>[2x]MEKKTIVLGVIGSDCHAVGNKILDHAFTNAGFNVVNIGVLSPQENFIKAAIETKADAILVSSLYGQGEIDCKGLRQKCDEAGLEGILLYVGGNIVVGKQHWPDVEKRFKDMGYDRVYAPGTPPEVGIADLKKDLNIE;>MELKNKKWTDEEFHKQREEVLQQWPTGKEVDLQEAVDYLKKIPAEKNFAEKLVLAKKKGITMAQPRAGVALLDEHIELLRYLQDEGGADF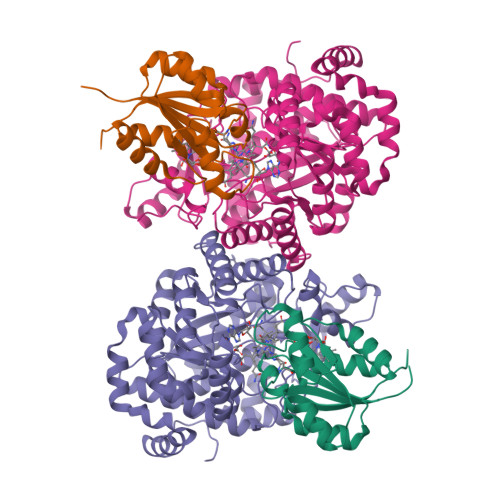LPSTIDAYTRQNRYDECENGIKESEKAGRSLLNGFPGVNHGVKGCRKVLEAVNLPLQARHGTPDSRLLAEIIHAGGWTSNEGGGISYNVPYAKNVTIEKSLLDWQYCDRLVGFYEEQGVHINREPFGPLTGTLVPPSMSNAVGITEALLAAEQGVKNITVGYGECGNMIQDIAALRCLEEQTNEYLKAYGYNDVFVTTVFHQWMGGFPQDESKAFGVIVTATTIAALAGATKVIVKTPHEAIGIPTKEANAAGIKATKMALNMLEGQRMPMSKELETEMAVIKAETKCILDKMFELGKGDLAIGTVKAFETGVMDIPFGPSKYNAGKMMPVRDNLGCVRYLEFGNVPFTEEIKNYNRERLQERAKFEGRDVSFQMVIDDIFAVGKGRLIGRPE[2x]> GSPDVRPVHGVHARMAEKMTLSHKEIPTAKASVEVICAELLRLRDRFVSAAPEITPFALTLRLLVIALKHNVILNSTWVDSGEGPQVHVHRGVHLGFGAATERGLLVPVVTDAQDKNTRELASRVAELITGAREGTLTPAELRGSTFTVSNFGALGVDDGVPVINHPEAAILGLGAIKPRPVVVGGEVVARPTMTLTCVFDHRVVDGA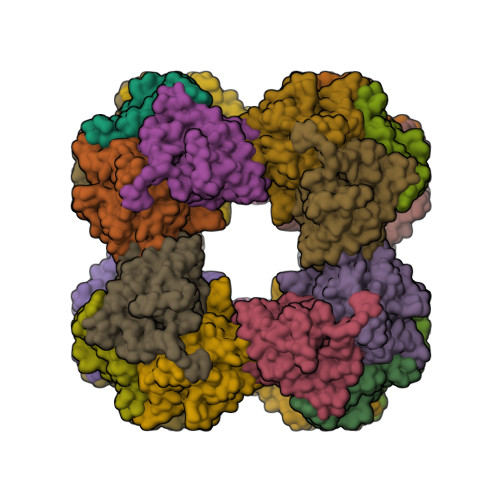QVAQFMCELRDLIESPETALLDL(4S)-4-hydroxy-L-proline | C5 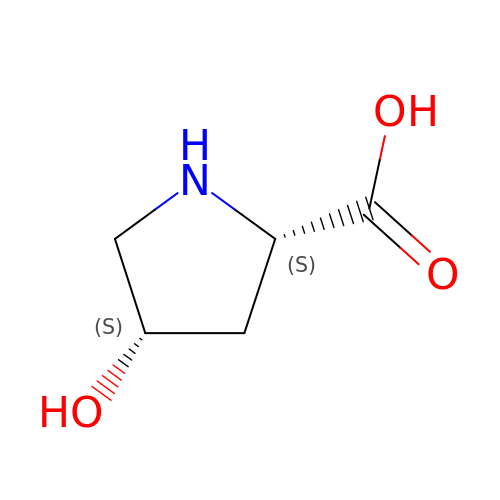H9 N O3 | PMMYEEVYMWASQN-IMJSIDKUSA-N> KETAAAKFERQHMDSSTSAASSSNYCNQMMKSRNLTKDRCKPVNTFVHESLADVQAVCSQKNVACKNGQTNCYQSYSTMSITDCRETGSSKYGNCAYKTTQ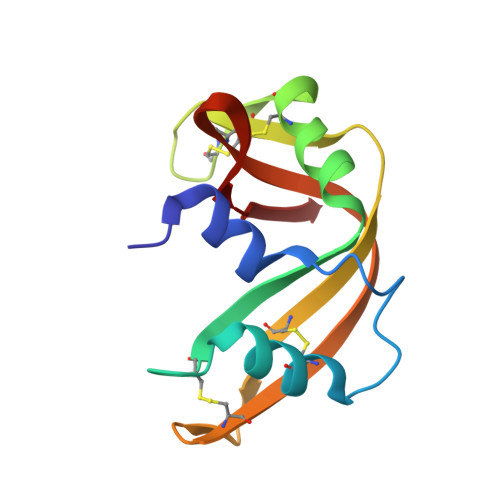ANKHIIVACEGNPYVPVHFDASV Fatty acid-binding proteins (FABPs) are involved in the uptake, metabolism and intracellular trafficking of fatty acids. Based on epidemiological studies and animal knockout models, the isoforms FABP4 and FABP5 were identified as potential diabetes and atherosclerosis targets. The aim of this study was to develop a dual FABP4/5 inhibitor and, to this end, high-throughput and fragment screens were conducted with X-ray crystallography as a follow-up method on those ligands that showed appreciable affinity and favorable physicochemical properties. Structure-based drug design (SBDD) based on initial hits from high-throughput and fragment screens yielded 216 ligand-bound structures of human FABP3, FABP4 and FABP5 isoforms, many of which were at resolutions of better than 1.2 Å.

However, a surprisingly large number of the ligands deviated from expectations. Next to possible human error (mis-labeling), prominent sources of deviations from expectation include side reactions of compounds, such as additions, eliminations, isomerizations, cyclizations and dimerizations.

>[3x]GSHMATVQQLEGRWRLVDSKGFDEYMKELGVGIALRKMGAMAKPDCIITCDGKNLTIKTESTLKTTQFSCTLGEKFEETTADGRKTQTVCNFTDGALVQHQEWDGKESTITRKLKDGKLVVECVMNNVTCTRIYEKVE>MELKNSISDYTEAEFVQLLKEIEKENVAATDDVLDVLLEHFVKITEHPDGTDLIYYPSDNRDDSPEGIVKEIKEWRA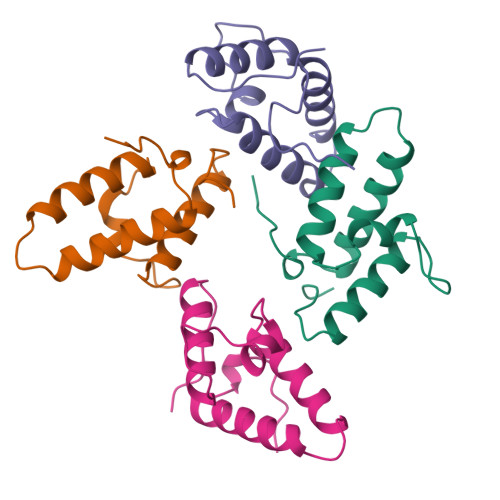ANGKPGFKQG[4x]>[6x]PAKKPYNKIVSHLLVAEPEKIYAMPDPTVPDSDIKALTTLCDLADRELVVIIGWAKHIPGFSTLSLADQMSLLQSAWMEILILGVVYRSLSFEDELVYADDYIMDEDQSKLAGLLDLNNAILQLVKKYKSMKLEKEEFVTLKAIALANSDSMHIEDVEAVQKLQDVLHEALQDY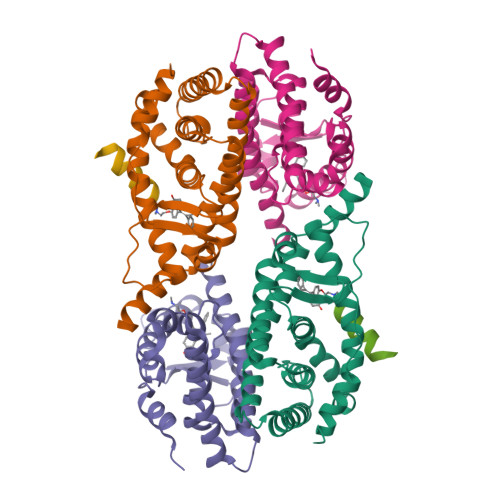EAGQHMEDPRRAGKMLMTLPLLRQTSTKAVQHFYNIKLEGKVPMHKLFLEMLEAKV;>[3x]TNMGLEAIIRKALMGKYDQWEE The hyperthermophilic L-ASNase from Thermococcus sibiricus (TsAI) was previously shown to exhibit high activity and thermostability and is promising for biotechnology. L-ASNase exerts its anticancer activity by hydrolyzing L-asparagine (L-Asn) in the bloodstream to L-aspartic acid and ammonia. The subunit of TsAI consists of two α/β domains: an N-terminal large domain (residues 1–184, consisting of twelve mixed β-sheets and four α-helices) and a C-terminal small domain (residues 207–331, consisting of three β-sheets and five α-helices) connected by an interdomain linker (residues 185–206). In the N-terminal domain, the active site pocket of TsAI includes residuesthat are highly conserved among all types of L-ASNases: Y22, S55, T56, T86, D87, K157, and T12, which initiates the reaction.

The mesophilic combination of highly conserved residues involved in catalysis and substrate-enzyme interaction was restored in TsAI by the double mutation D54G/T56Q (TsAID54G/T56Q) that resulted in a two-fold increase in activity. Superposition of TsAI and its mutant form TsAID54G/T56Q showed stability of the fold for these structures (the RMSD for the Cα atoms does not exceed 0.2 Å). The most significant difference between them was observed in the conformation of residues 51–57, where two substitutions occurred. The point mutation T56Q led to the formation of a hydrogen bond between Q56 and S15 side chains in TsAID54G/T56Q. At the same time, the D54G mutation destroyed the network of hydrogen bonds. Together, this led to a change in the conformation of this loop that was additionally fixed by the formation of a water-mediated hydrogen bond between the S55 and D62 side chains. Moreover, the part of this loop (residues 52 and 53) has no electron density, confirming the increased mobility of this region. Overall, the experimental data show that the increased flexibility of the loop M51-L57 due to mesophilic-like replacement D54G/T56Q is the key structural difference between TsAI forms. The significance of loop mobility for TsAI enzymatic activity is confirmed by the two-fold increase in activity in the mutant form after disruption of “redundant” hydrogen bonds. On the other hand, TsAID54G/T56Q exhibits a sharper temperature optimum curve and increased time-dependent loss of activity compared with the wild-type TsAI.

> MKKLLIIGTGGTIASAKTEQGYKSVLKIDEILKLAKIKLENGYKIDSTNIMNIGSQLIHPEDWEIIAKEVFKALDDYDGIIITHGTDTLAYTASMLSFMIKNPNKPIVLTGSMLPITENGSDAPRNIRTAIKFAMEDVAGVFVAFMDKIMLGCRTSKVRTLGLNAFMSINYPDVAYVKGEKILYNIPKEKFQPNGSPELDTKYEPRVVVLRVTPGLGGEIIDAVLDAGYKGIVLEGYGAGGLPYRKSNLLSKIKEITPKIPVIMTTQALYDGVDMRKYEVGRKALETGIIPAKDMTKEATITKLMWALGHTKDVEKIREIMHTNYVNEIKS> MNLNSIPAFDDNYIWVLNDEAGRCLIVDPGDAEPVLNAIAANNWQPEAIFLTHHHHDHVGGVKELVEKFPQ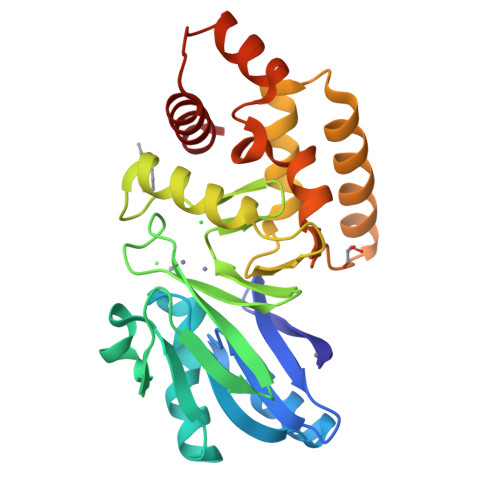IVVYGPQETQDKGTTQVVKDGETAFVLGHEFSVIATPGHTLGHICYFSKPYLFCGDTLFSGGCGRLFEGTASQMYQSLKKLSALPDDTLVCCAHEYTLSNMKFALSILPHDLSINDYYRKVKELRAKNQITLPVILKNERQINVFLRTEDIDLINVINEETLLQQPEERFAWLRSKKDRF(5S)-5-{[(2R,3S,4R,5R)-5-(6-amino-9H-purin-9-yl)-3,4-dihydroxytetrahydrofuran-2-yl]methyl}-N~6~-carbamimidoyl-L-lysine 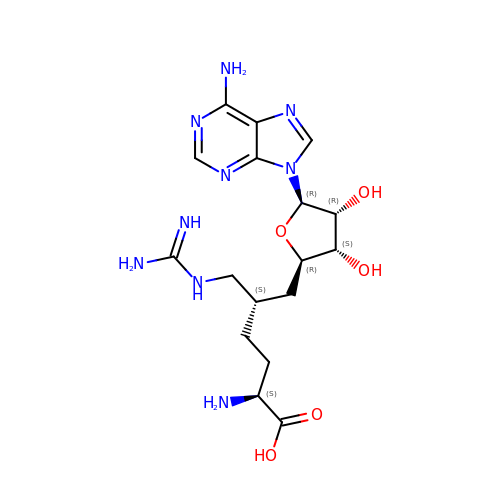| C17 H27 N9 O5 | PRQKNHVENSAKGM-TVDBPQCTSA-N Rhodotorula dairenensis β-fructofuranosidase is a highly glycosylated enzyme with broad substrate specificity that catalyzes the synthesis of 6-kestose and a mixture of the three series of fructooligosaccharides (FOS), fructosylating a variety of carbohydrates and other molecules as alditols. RdINV subunit is composed of two domains, similar to the rest of the reported fungal β-fructofuranosidases within GH32. The β-propeller catalytic domain contains residues 185 to 487 and is constituted by five blades (I-V), each involving four antiparallel β-strands (ABCD) with a “W” topology. The β-sandwich domain, extending from residue 495 to 673, is composed of twelve β-sheets ordered in two six-stranded clusters of antiparallel β-strands.

To analyze its hydrolytic activity, the inactivated D188A-RdINVΔ21–139 mutant was deglycosylated, crystallized and used for soaking experiments with different sugars, including fructose, sucrose, 1-kestose, raffinose or nystose, and, also, ternary complexes with fructose and palatinose, trehalose or hydroxytyrosol have also been pursued. However, only complexes of this truncated variant with fructose, sucrose or raffinose were obtained, the crystals belonging to the P21 space group with two complete dimers within the asymmetric unit that are essentially similar. To obtain D188A-RdINVΔ21–139 fructose complex, crystals were grown in 18% PEG 3350, 0.2 M MgCl2, 0.1 M Bis-Tris pH 5.5 solution (1:1 rate) in the presence of 20 mM fructose. Diffraction data of D188A-RdINVΔ21–139 in complex with fructose, sucrose and raffinose were collected at the ALBA synchrotron station (Barcelona, Spain), being indexed in the P21 space group with four molecules in the asymmetric unit, at 1.86 Å, 2.38 Å and 2.27 Å, respectively. The crystal complexes show clear electron density at the active site that allows unambiguous ligand modeling. Remarkably, a net of well-ordered water molecules is found in all complexes, contributing to substrate binding. Moreover, the Bis-Tris molecule shows one of its hydroxyl groups very close to the fructose and, thus, is in a proper position to act as an acceptor substrate in a putative transfructosylating reaction. This is consistent with and illustrates the previously reported fructose transference activity on various polyols.

>[4x]MKFTLLSVVAIAAAASDSYAAPAASSLAGPVTTGVFSAVSAIPSFATNLSGQVASATSTVLSGSTASGSSATAAPSASASGASSMQSMASSLSGSAFSPSSMMPIASGNMTMPNMTSSASASSAASTATGVAGGAGSNSSSSCAPTSLPASATELPTTVPTGTVITGDYTGSYRPQVHYSPPKGFMNAPNGCHRDRNGTYHLYYQYNPLEYVAGNQHWGHATSDDLYHWTNQPIAIFPPNSTSQVFSGSAVLDPNNTSGFFPNTTDGVVAVYTLNTPTLQVQEVAYSTDGGYNFTPYENNPVLSVGSNQFRDPKVFWYEDHWVMAVAAANDFTIEIYTSPNLTSWTFASNFTHHGLLGLAYECPNLVQVPFQDDPSKSAWLMYISINPGAPLGGSVGQYFPGDFNGTHFVAYDSAARIADFAKDNYASQWFADTENGESISIAWASNWQYTQQVPTSAQAFRSAMSLPRRNYLTNITRLGWDLVSLPYDLSPVVGPSLLSSSEANSTADVDFTNVTSNAVWFSLNVTLPDAAIQNASLISADASINITFLPSTKCSSSSGSGSDSPAATLTYFYAGLTNGALALTRPAASSSWGAENPFFTDKFSYTLVDPLTSLVGVFDRSMLEVFVNEGAHSATMLVFPDSPVGSMKVATGGLPEGTQVNLQVNGLESTWQSS>[4x]G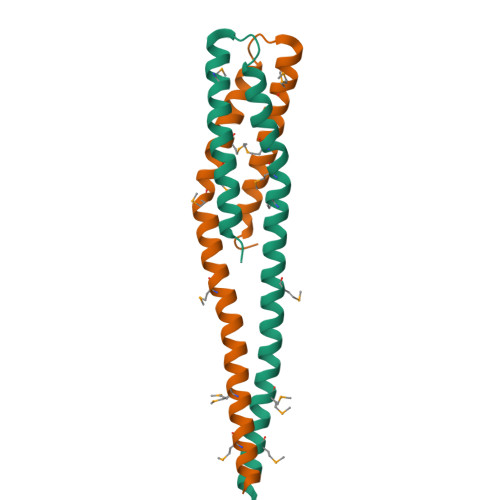ASHAAILEESMHARDQLMEQNFALDKARQEAEMAVHARNDFLAVMNHEMRTPMHAIISLSSLLLETELSPEQRVMIETILKSSNLVATLISDVLDLSRLED2,6 DIMETHOXYBENZAMIDOBORONIC ACID | C10 H14 B N 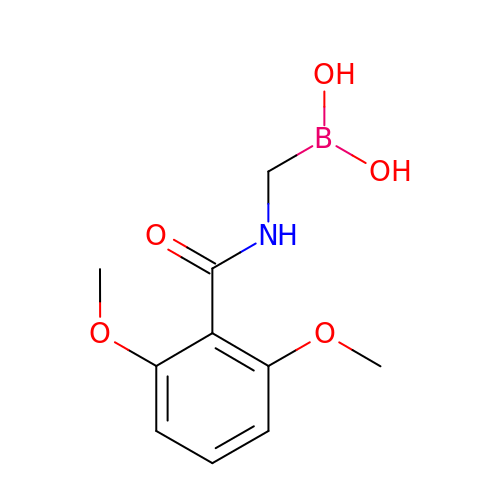O5 | SXURQNHWSSEFLG-UHFFFAOYSA-N> SMGKAPVDPECTAKVGKAHVYCEGNDVYDVMLNQTNLQFNNNKYYLIQLLEDDAQRNFSVWMRWGRVGKMGQHSLVACSGNLNKAKEIFQKKFLDKTKNNWEDREKFEKVPGKYDMLQMDYATNTQDEEETKKEESLKSPLKPESQLDLRVQELIKLICNVQAMEEMMMEMKYNTKKAPLGKLTVAQIKAGYQSLKKIEDCIRAGQHGRALMEACNEFYTRIPHDFGLRTPPLIRTQKELSEKIQLLEALGDIEIAIKLVKTELQSPEHPLDQHYRNLHCALRPLDHESYEFKVISQYLQSTHAPTHSDYTMTLLDLFEVEKDGEKEAFREDLHNRMLLWHGSRMSNWVGILSHGLRIAPPEAPITGYMFGKGIYFADMSSKSANYCFASRLKNTGLLLLSEVALGQCNELLEANPKAEGLLQGKHSTKGLGKMAPSSAHFVTLNGSTVPLGPASDTGILNPDGYTLNYNEYIVYNPNQVRMRYLLKVQFNFLQLW

Human PARP2/ARTD2 is an ADP-ribosyltransferase which, when activated by 5′-phosphorylated DNA ends, catalyses poly-ADP-ribosylation of itself, other proteins and DNA. In the nucleus, the main enzymes carrying out poly-ADP-ribosylation are poly(ADP-ribose) polymerase 1 (PARP1) and PARP2. These enzymes bind to the damaged DNA and subsequently generate poly-ADP-ribose (PAR) chains that act as recruitment signals for a range of DNA repair factors. The WGR domain of PARP2 has been shown to be key to DNA damage recognition.

We determined a PARP2 crystal structure consisting of the WGR domain and catalytic fragment (PARP2WGR-RD-ART; residues 90-583) in complex with an activating double-stranded oligonucleotide mimicking a damaged DNA. The structure was obtained by using a multicrystal approach where 26 small datasets were merged in order to achieve a complete dataset at 2.8 Å resolution. The asymmetric unit contains one PARP2WGR-RD-ART molecule with one dsDNA (DNA-1), while the biological unit has an apparent 2:2 stoichiometry in solution. The complex is formed by two dsDNA oligonucleotides joined together at the phosphorylated ends by two flanking proteins. The WGR domain detects the phosphorylated DNA end coordinated by Trp151, Lys130, Lys183 and Tyr201. Tyr201 (Phe638 in PARP1) forms a hydrogen bond with the phosphate, whereas Arg153 and Asn127 (Gly565 in PARP1) interact with the N-1 nucleotide from the 3′ end and bridge the connection to Gly314 of the RD domain. Interestingly, in addition to binding to the phosphorylated DNA break by the WGR domains, the crystal symmetry showed that the catalytic site was also in contact with the DNA, namely the unphosphorylated end, where the last A-T base pair is opened up. The 3′-adenosine ribose interacts with the helix lining the active site and its ribose makes only one hydrogen bond to Asp396, while the 5′-thymine binds to the active site and locates in the nicotinamide binding site between two tyrosine side chains. Upon DNA binding, helix α5, covering the active site in the inactive conformation, is divided into two parts at Gly338, and the helices are completely reorganized. Subsequently, the catalytic transferase domain moves ~11 Å away from the DNA and it is rotated and translated implying mobility in solution.>[6x]XGEIAKSLKEIA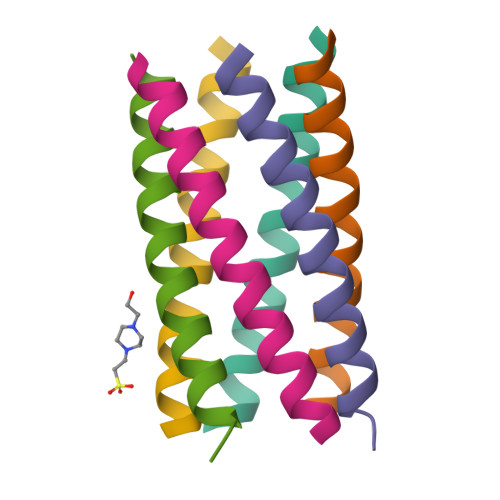KSLKEIAWSLKEIAKSLKG>SMADGNEDLRADDLPGPAFESYESMELACPAERSGHVAVSDGRHMFVWGGYKSNQVRGLYDFYLPREELWIYNMETGRWKKINTEGDVPPSMSGSCAVCVDRVLYLFGGHHSRGNTNKFYMLDSRSTDRVLQWERIDCQGIPPSSKDKLGVWVYKNKLIFFGGYGYLPEDKVLGTFEFDETSFWNSSHPRGWNDHVHILDTETFTWSQPITTGKAPSPRAAHACATVGNRGFVFGGRYRDARMNDLHYLNLDTWEWNELIPQGICPVGRSWHSLTPVSSDHL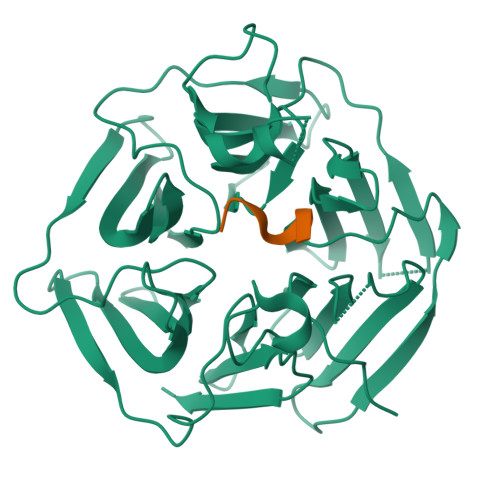FLFGGFTTDKQPLSDAWTYCISKNEWIQFNHPYTEKPRLWHTACASDEGEVIVFGGCANNLLVHHRAAHSNEILIFSVQPK[2x];>[2x]PPPMAGG>GNNRALINDKLASLQYNPKTVMVFNGTSISNIDLPAEERFDDSTYIVMTREKCSYEADFDIAVPSAYEDVTYPGALLVASNDLLDGKPQELAVDKDRVNITVDLPGATDISFKVVPTFANVRAGINDILSKWFDSHGGEWSLPANFQYSSSLVYDENELMLKFGCDISYLKQKLSIDFSSTRAEKKSVYLIRFKQIFYSVSAERPAKPADIFAESTTWEDLARAGISEEHPPLFVKNVQYGRQIFLKFESKLSSTELETTIKGTCSKDGLKIDANASAALKEKLSQIDVSIVVHGGSEAVYNGLSLNSMDDVQKINRIIWDNTLLSRTNTAAPLNYYTVFLKDGVSAGVHGTTEYVAEKTERYSGGEIRLEHSGWYVARFTVTWDEISYE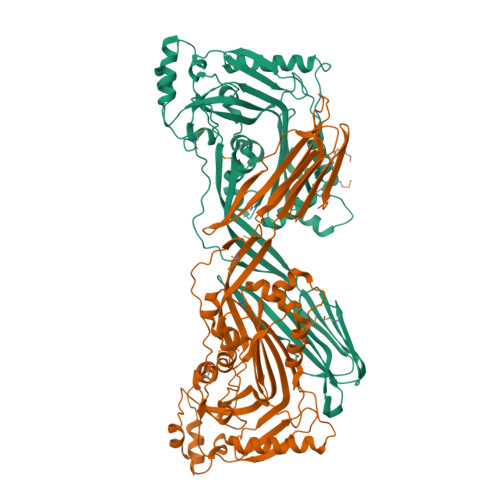NGLKVIRHKGWEGNGKDRTAPFSTTIPLRGNARNISIKTEGCTGLAWEWWRTSGYKVGRALVPLRTVSIGGTTLHQTFSMTPAD[2x]> HIEGYECQPIF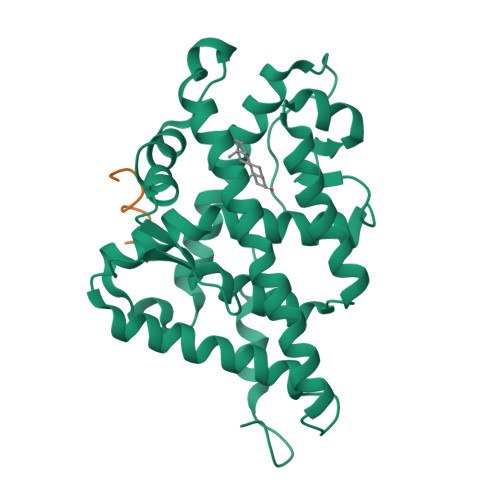LNVLEAIEPGVVCAGHDNNQPDSFAALLSSLNELGERQLVHVVKWAKALPGFRNLHVDDQMAVIQYSWMGLMVFAMGWRSFTNVNSRMLYFAPDLVFNEYRMHKSRMYSQCVRMRHLSQEFGWLQITPQEFLCMKALLLFSIIPVDGLKNQKFFDELRMNYIKELDRIIACKRKNPTSCSRRFYQLTKLLDSVQPIARELHQFTFDLLIKSHMVSVDFPEMMAEIISVQVPKILSGKVKPIYFHTQ;> HKKLLQLLT>SVKLAGNSSLCPVSGWAIYSKDNSVRIGSKGDVFVIREPFISCSPLECRTFFLTQGALLNDKHSNGTIKDRSPYRTLMSCPIGEVPSPYNSRFESVAWSASACHDGINWLTIG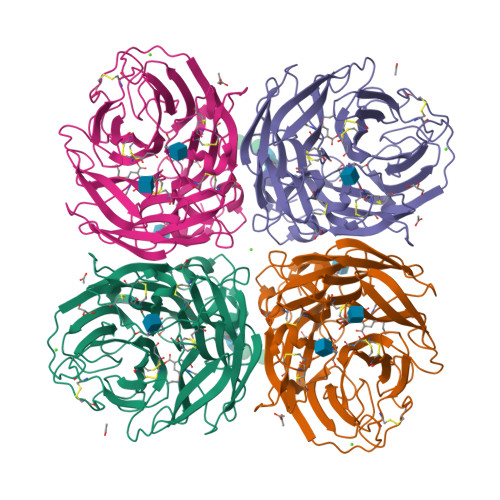ISGPDNGAVAVLKYNGIITDTIKSWRNNILRTQESECACVNGSCFTVMTDGPSNGQASYKIFRIEKGKIVKSVEMNAPNYHYEECSCYPDSSEITCVCRDNWHGSNRPWVSFNQNLEYQIGYICSGIFGDNPRPNDKTGSCGPVSSNGANGVKGFSFKYGNGVWIGRTKSISSRNGFEMIWDPNGWTGTDNNFSIKQDIVGINEWSGYSGSFVQHPELTGLDCIRPCFWVELIRGRPKENTIWTSGSSISFCGVNSDTVGWSWPDGAELPFTIDK[2x]>[10x]GSHMGGIEVLDVKTGDDSITQIEAFLNPRMGVNDETNTWYGFSEQVTVATARETDRPPKEQMPYYSCARIPLPLLNEDMTCNTLLMWEAVSVKTEVIGSNTLMNVHDYMTRTDNGVGHPVVGSTYHMFAVGGEPLDLQGIQQSHLVQYPEGLIVPKSVTDVTAKIQCLDPSAKAKLDKDGKYPIETWSPDPSRNENTRYFGNYYGGLTTPPVLTFTNTVTTILLDENGVGPLCKGDGLFLSCCDVMGWFTAGSGTHQRFRGLPRYFNVQLRKRAVRN

Polyomaviruses are small double-stranded DNA (dsDNA) viruses with a circular genome of approximately 5,000 bp. All glycan-binding polyomaviruses analyzed to date engage oligosaccharide (glycan) structures featuring terminal sialic acids that in mammals are usually presented either on gangliosides, which are molecules composed of a glycosphingolipid, i.e., a ceramide and an oligosaccharide, or on glycoproteins, which contain mostly complex and branched oligosaccharides attached to amino acids during co- and posttranslational modification steps. These sialylated glycan structures interact with loop regions at the outer margin of the major capsid protein VP1, at the apical surface of the polyomavirus capsid, as revealed by X-ray crystallography and cryoelectron microscopy. The VP1 surface exhibits an astonishing plasticity, providing virus-specific interactions for a range of Neu5Ac linkage types and further specific characteristics of Neu5Ac-containing glycans.

In the crystal structure of the HPyV12 VP1 pentamer in complex with 3′SLN, the Neu5Ac moiety of the linear trisaccharide is engaged in a binding site mainly formed by the BC2 loop of one VP1 monomer. The Neu5Ac N-acetyl group inserts into a shallow cavity, forming a hydrogen bond between its amide group and residue T69. Additional, nonpolar interactions involve the methyl group and residues P79 and H128 of the counterclockwise (ccw) VP1 monomer. Finally, the N-acetyl carbonyl oxygen forms direct and water-mediated hydrogen bonds with the backbone amide groups of R78 and T72, respectively. The Neu5Ac glycerol chain forms hydrogen bonds with the side chain of R133 from the ccw DE loop and with the backbone amine of residue V70. On the other side of the BC2 loop, the Neu5Ac C-4 hydroxyl group interacts with the protein backbone. The Neu5Ac carboxylate group is not involved in any direct interactions with VP1, only forming a water-mediated hydrogen bond with the side chain of residue Q83. Cα atoms of the BC2 loop (residues 67 to 82) from the liganded HPyV12 VP1 structure superpose with the respective residues of the native structure with an RMSD of 0.3 Å (55), indicating that the Neu5Ac docks into a preformed binding pocket within the BC2 loop and that no conformational changes occur upon ligand binding. Well-defined electron density was observed for the Neu5Ac ring in all 10 VP1 binding sites of the asymmetric unit, and in some sites the Gal ring could also be unambiguously built into the electron density. The interactions used by HPyV12 to engage terminal Neu5Ac are strikingly similar to those used by TSPyV.2-amino-1-(4-fluorophenyl)ethan-1-one 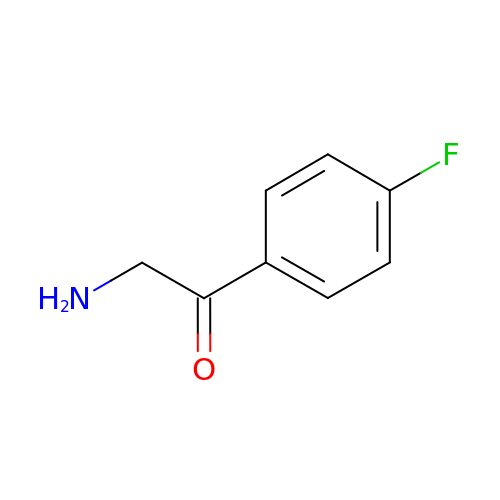| C8 H8 F N O | HLYXSMQJWZMANE-UHFFFAOYSA-N>[2x]GPGSEFGEVVDCHLSDMLQQLHSVNASKPSERGLVRQEEAEDPACIPIFWVSKWVDYSDKYGLGYQLCDNSVGVLFNDSTRLILYNDGD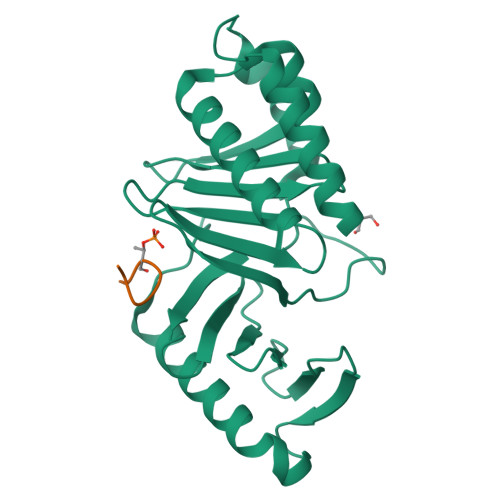SLQYIERDGTESYLTVSSHPNSLMKKITLLKYFRNYMSEHLLKAGANITPREGDELARLPYLRTWFRTRSAIILHLSNGSVQINFFQDHTKLILCPLMAAVTYIDEKRDFRTYRLSLLEEYGCCKELASRLRYARTMVDKLLSSR;>ESCFTNAAFSSTPKK[2x]> MASVHGTTYELLRRQGIDTVFGNPGSNELPFLKDFPEDFRYILALQEACVVGIADGYAQASRKPAFINLFSAAGTGNAMGALSNAWNSHSPLIVTAGQQTRAMIGVEALLTNVDAANLPRPLVKWSYEPASAAEVPHAMSRAIHMASMAPQGPVYLSVPYDDWDKDADPQSHHLFDRHVSSSVRL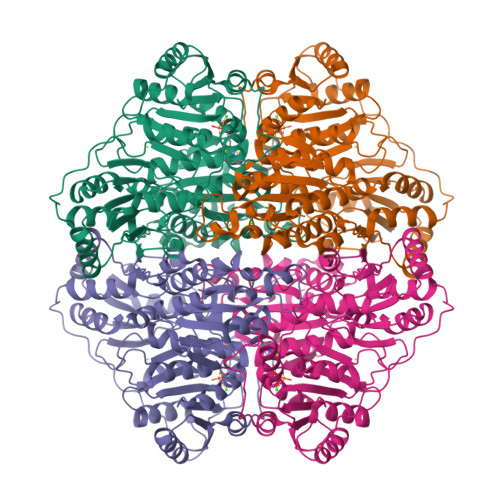NDQDLDILVKALNSASNPAIVLGPDVDAANANADCVMLAERLKAPVWVAPSAPRCPFPTRHPCFRGLMPAGIAAISQLLEGHDVVLVIGAPVFRYHQYDPGQYLKPGTRLISVTCDPLEAARAPMGDAIVADIGAMASALANLVEESSRQLPTAAPEPAKVDQDAGRLHPETVFDTLNDMAPENAIYLNESTSTTAQMWQRLNMRNPGSYYFCAAGGLGFALPAAIGVQLAEPERQVIAVIGDGSANYSISALWTAAQYNIPTIFVIMNNGTYGALRWFAGVLEAENVPGLDVPGIDFRALAKGYGVQALKADNLEQLKGSLQEALSAKGPVLIEVSTVSPVKHHHHHH5-METHOXY-2-[(4-PHENOXYPHENYL)AMINO]BENZOIC ACID | C20 H17 N 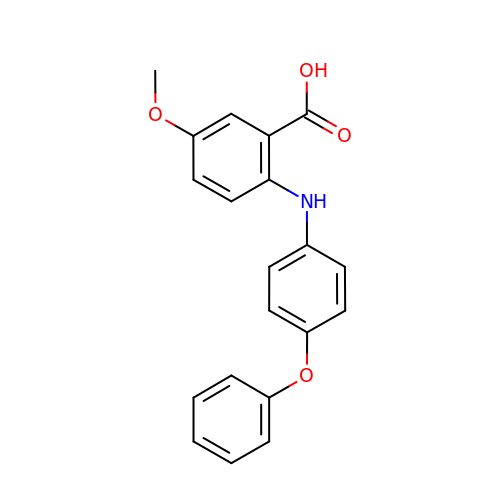O4 | YJRDHMUPONVWTE-UHFFFAOYSA-N>[4x]MPNYKLTYFNMRGRAEIIRYIFAYLDIQYEDHRIEQADWPEIKSTLPFGKIPILEVDGLTLHQSLAIARY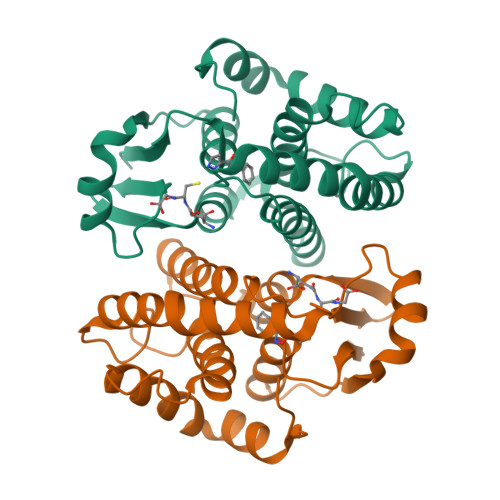LTKNTDLAGNTEMEQCHVDAIVDTLDDFMSCFPWAEKKQDVKEQMFNELLTYNAPHLMQDLDTYLGGREWLIGNSVTWADFYWEICSTTLLVFKPDLLDNHPRLVTLRKKVQAIPAVANWIKRRPQTKL1-methyl-~{N}-(1-thiophen-2-ylcarbonyl-3,4-dihydro-2~{H}-quinolin-6-yl)-~{N}-[2,2,2-tris(fluoranyl)ethyl]indole-4-sulfonamide | C25 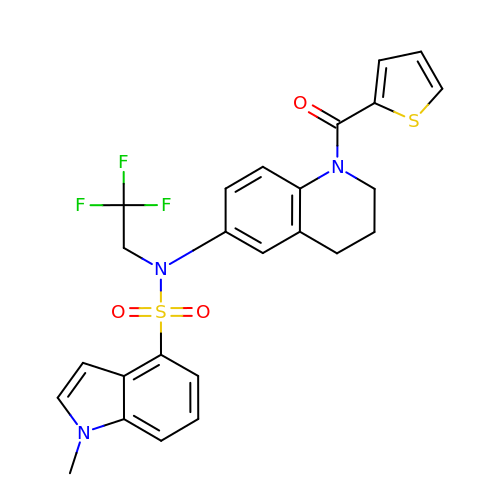H22 F3 N3 O3 S2 | MGKISJPOEOHZCS-UHFFFAOYSA-N> MATEVTFFDELKIDN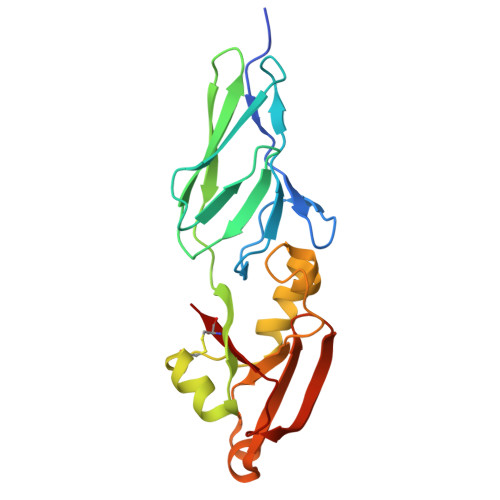KVDIIGNNVRGELPNIWLQYGQFKLKASGGDGTYSWYSENTSIATVDASGKVTLNGKGSVVIKATSGDKQTVSYTIKAPSYMIKVDKQAYYADAMSICKNLLPSTQTVLSDIYDSWGAANKYSHYSSMNSITAWIKQTSSEQRSGVSSTYNLITQNPLPGVNVNTPNVYAVCVE> D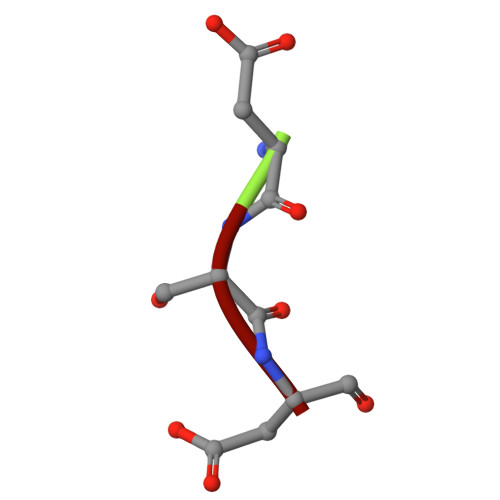SD> SMAENREPRGAVEAELDPVEYTLRKRLPSRLPRRPNDIYVNMKTDFKAQLARCQKLLDGGARGQN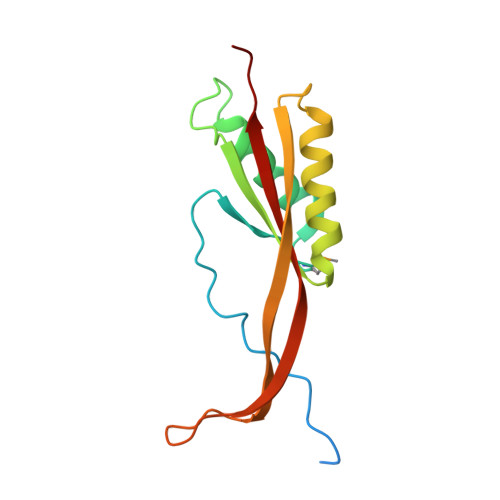ACSEIYIHGLGLAINRAINIALQLQAGSFGSLQVAANTSTVELVDELEPETDTREPLTRIRNNSAIHIRVFRVTPK> MIHSLFLINCSGDIFLEKHWKSVVSQSVCDYF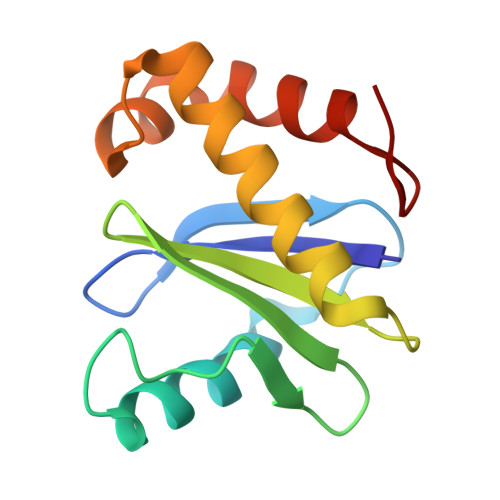FEAQEKAADVENVPPVISTPHHYLISIYRDKLFFVSVIQTEVPPLFVIEFLHRVADTFQDYFGECSEAAIKDNVVIVYELLEEMLDNGFPLA> MGSSHHHHHHSSGLVPRGSHMSPSPVPGSQNVPAPAVKKISQYACQRRTTLNNYNQLFTDALDILAENDELRENEGSCLAFMRASSVLKSLPFPITSMKDTEGIPCLGDKVKSIIEGIIEDGESSEAKAVLNDERYKSFKLFTSVFGVGLKTAEKWFRMGFRTLSKIQSDKSLRFTQMQKAGFLYYEDLVSCVNRPEAEAVSMLV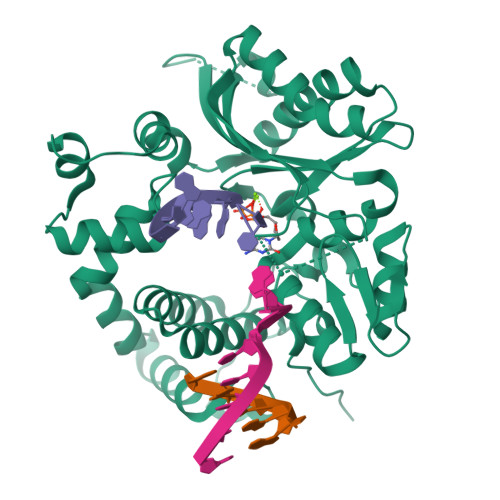KEAVVTFLPDALVTMTGGFRRGKMTGHDVDFLITSPEATEDEEQQLLHKVTDFWKQQGLLLYCDILESTFEKFKQPSRKVDALDHFQKCALILKLDHGRVHSEKSGQQEGKGWKAIRVDLVMCPYDRRAFALLGWTGSRQFERDLRRYATHERKMMLDNHALYDRTKRVFLEAESEEEIFAHLGLDYIEPWERNA> ESPFVSNPGNITGARGLTGTLRCQLQVQGE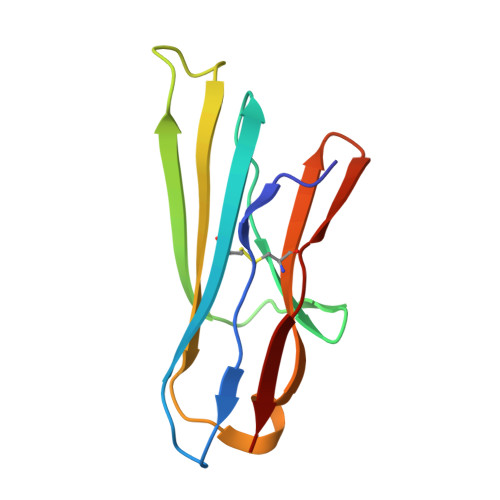PPEVHWLRDGQILELVDSTQTQVPLGEDEQGDWIVASQLRITSLQLSDTGQYQCLVFLGHQTFVSQPGYVRL> MQTFTAREYLKIDIANNYGLDKEDWDDRIAWFDKNENNLLNLVREAEEPALFYAGVKAWMDVKEGKPIGYPVALDATSSGLQILACLTGDRRAAELCNVVNYRDESGKVKRRDAYTVIYNKMLNTLGKGARIKRNDCKQAIMTALYGSEAKPKEVFGEGIMLNVFESTMNVEAPAVWELNKFWLQCGNPEAFVYHWVMPDGFNVYIKVMVNEVETVHFLDKPYDCVRKVQGTEEKTRMLSANT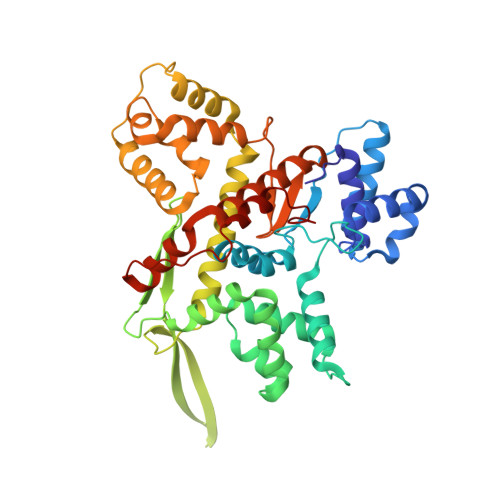THSIDGLVVRELVRRCDYDKNQIEYIKALCNGEAEYKASEKNYGKAMELWGYYEKTGFLTARIFDYLDSETIKLVNTQDILDLIESMPKKPFHVLTVHDCFRCLPNYGNDIRRQYNNLLATIAKGDLLSFIMSQVIGQEVTIGKLDPTLWEDVLETEYALS> MRERPHTSGHHGAGEARATAPSTVSPYGPEARAELSSRLTTLRNTLAPATNDPRYLQACGGEKLNRFRDIQCRRQTAVRADLNANYIQVGNTRTIACQYPLQSQLESHFRMLAENRTPVLAVLASSSEIANQRFGMPDYFRQSGTYGSITVESKMTQQVGLGDGIMADMYTLTIREAGQKTISVPVVHVTNWPDQTAVSSEVTKALASLVDQTAETKRNMYESKGSSAVADDSKLRPVIHCRAGVGRTAQLIGAMCMNDSRNSQLSVEDMVSQMRVQRNGIMVQKDEQLDVLIKLAEGQGRPLLNS

Catalysis by protein tyrosine phosphatases (PTPs) relies on the motion of a flexible protein loop (the WPD-loop) that carries a residue acting as a general acid/base catalyst during the PTP-catalyzed reaction. The classical PTPs hydrolyze only phosphotyrosine (pTyr) residues of polypeptide substrates, while the dual-specific subfamily members (DSPs) also dephosphorylate phosphoserine (pSer) and phosphothreonine (pThr) residues. All PTPs share the conserved signature motif HCX5R(S/T) forming the P-loop, which includes the nucleophilic cysteine and a conserved arginine, which, along with backbone amides, binds substrate and provides transition-state stabilization. In addition to the P-loop, PTPs share an aspartic acid that protonates the leaving group in the first chemical step and then, as a carboxylate, activates the nucleophilic water molecule in the second step. Closure of the WPD-loop moves the conserved Asp residue about 9 Å into the position needed for catalysis.

Structures were obtained of the PTP1B T177G and YopH G352T ligand-free enzymes and in complex with vanadate. In both ligand-free structures, the WPD-loops are observed in the closed position. This is in contrast to the typical observation of this loop in the open, noncatalytic position in crystal structures of these and other PTPs lacking a bound oxyanion. There has been no X-ray structure reported of ligand-free WT YopH with its loop in the closed conformation. Particularly, for the YopH variant, the closed conformation found suggests the G352T mutation has shifted the equilibrium of the ligand-free enzyme to favor the closed conformation. The G352T substitution in YopH introduces a new 3.3 Å hydrogen bond between the side chain of T352 and the backbone carbonyl of M328 in both the ligand-free and vanadate-bound structures, stabilizing the loop-closed conformation. If this hydrogen bond is only present, or is tighter, in the loop-closed conformation, it would rationalize the presence of this conformation in the ligand-free structure in contrast to the native enzyme. We were unable to obtain a crystal structure of a loop-open conformation of the mutant, and interactions of T352 in that conformation are unknown. The difference between them is nearly identical to the previous report, and this smaller difference in YopH relative to PTP1B gives rise to its narrower pH profile. Its G352T variant shows a much broader pH-rate profile than WT, with a kinetic pKa of the nucleophilic Cys residue lower by about a full unit. Thus, the different pH dependency of the G352T variant arises not from substantial alteration of the thermodynamic pKa of the thiol group of the cysteine side chain but predominantly from altered dynamic properties that affect the factors described in the Introduction, which distort the kinetic pKa values from their thermodynamic values and affect the pH dependency of catalysis.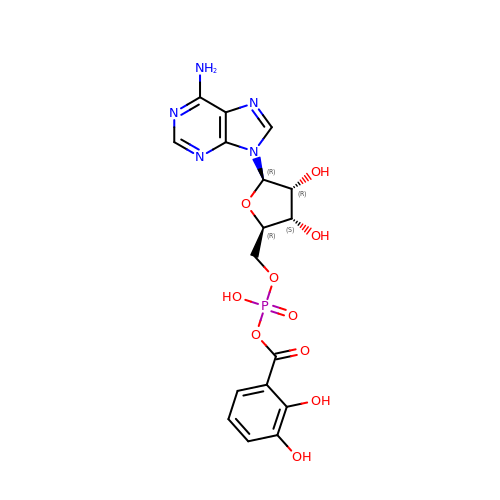5'-O-[(S)-[(2,3-dihydroxybenzene-1-carbonyl)oxy](hydroxy)phosphoryl]adenosine | C17 H18 N5 O10 P | ULPVJDOMCRTJSN-RVXWVPLUSA-N>SEFGEKQRV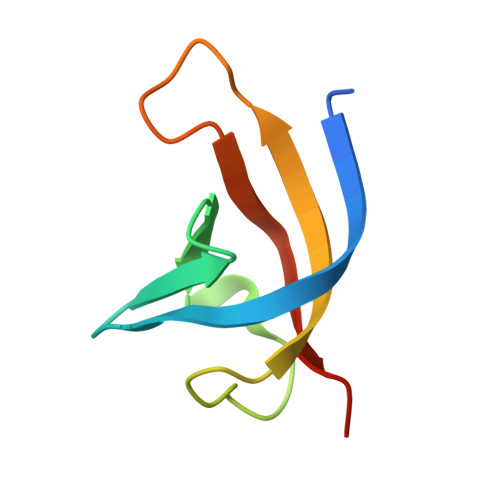FTGIVTSLHDYFGVVDEEVFFQLSVVKGRLPQLGEKVLVKAAYNPGQAVPWNAVKVQTLSNQP[2x]> SALLEKIEKEAERLLDKDEAKLLILAEKF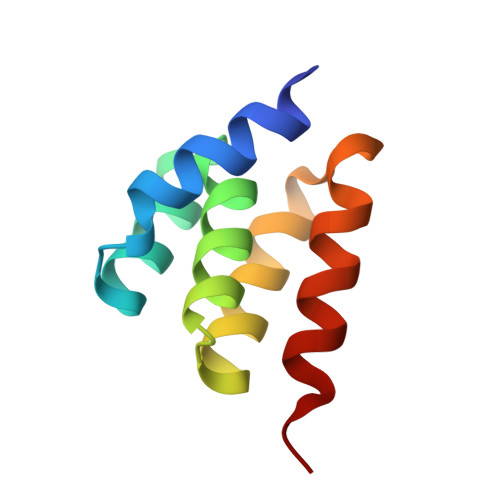SGYAPACLLALVRQGADSLSLLIALEILLKVLTPENEPIILLGLKAILEKE>V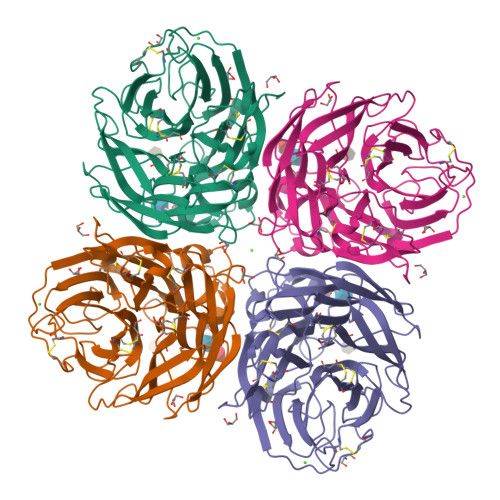ILTGNSSLCPISGWAIYSKDNGIRIGSKGDVFVIREPFISCSHLECRTFFLTQGALLNDKHSNGTVKDRSPYRTLMSCPVGEAPSPYNSRFESVAWSASACHDGMGWLTIGISGPDNGAVAVLKYNGIITDTIKSWRNNILRTQESECACVNGSCFTIMTDGPSNGQASYKILKIEKGKVTKSIELNAPNYHYEECSCYPDTGKVMCVCRDNWHGSNRPWVSFDQNLDYQIGYICSGVFGDNPRPNDGTGSCGPVSSNGANGIKGFSFRYDNGVWIGRTKSTSSRSGFEMIWDPNGWTETDSSFSVRQDIVAITDWSGYSGSFVQHPELTGLDCMRPCFWVELIRGQPKENTIWTSGSSISFCGVNSDTVGWSWPDGAELPFSI[2x]> GPAIASEFSSLPSYAAFATAQEAYEQAVANGDSEVVLKKLKKSLNVAKSEFDRDAAMQRKLEKMADQAMTQMYKQARSEDKRAKVTSAMQTMLFTMLRKLDNDALNNIINNARDGCVPLNIIPLTTAAKLMVVIPDYNTYKNTCDGTTFTYASALWEIQQVVDADS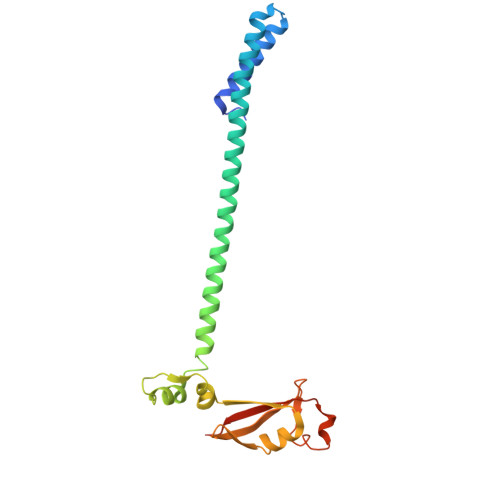KIVQLSEISMDNSPNLAWPLIVTALRANSAVKLQ>VDFKLSPSQLEARRHAQAFANTVLTKASAEYSTQKDQLSRFQATRPFYREAVRHGLIKAQVPIPLGGTMESLVHESIILEELFAVEPATSITIVATALGLMPVILCDSPSLQEKFLKPFISGEGEPLASLMHSEPNGTANWLQKGGPGLQTTARKVGNEWVISGEKLWPSNSGGWDYKGADLACVVCRVSDDPSKPQDPNVDPATQIAVLLVTRETIANNKKDAYQILGEPELAGHITTSGPHTRFTEFHVPHENLLCTPGLKAQGLVETAFAMSAALVGAMAIGTARAAFEEALVFAKSDTRGGSKHIIEHQSVADKLIDCKIRLETSR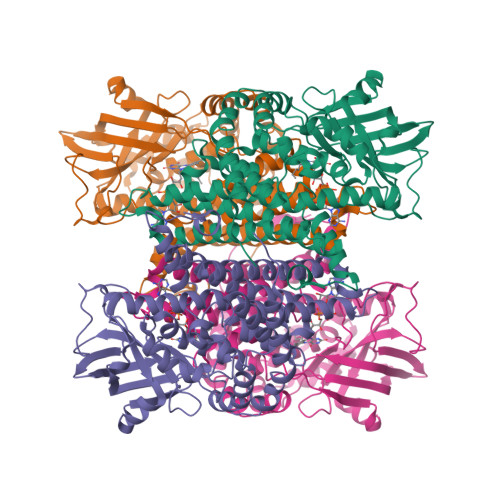LLVWKAVTTLEDEALEWKVKLEMAMQTKIYTTDVAVECVIDAMKAVGMKSYAKDMSFPRLLNEVMCYPLFDGGNIGLRRRQMQRVMALEDYEPWAATYGSSKVDKSRL[4x]(3R,5R)-7-[2-(4-fluorophenyl)-4-{[(1S)-2-hydroxy-1-phenylethyl]carbamoyl}-5-(1-methylethyl)-1H-imidazol-1-yl]-3,5-dihydroxyheptanoic 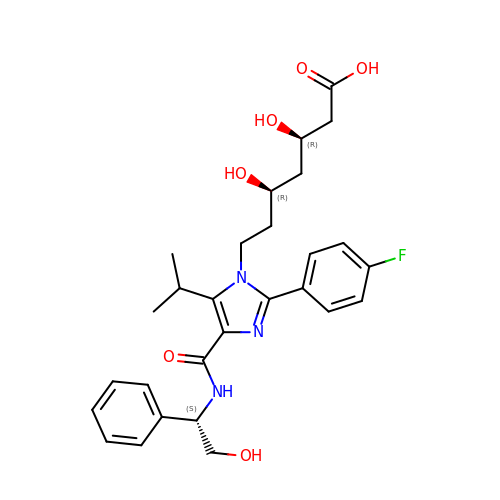acid | C28 H34 F N3 O6 | YBLASZBVZVCRFU-DNVJHFABSA-N> MGVVEEAHNVKVIGSGEATIVLGHGFGTDQSVWKHLVPHLVDDYRVVLYDNMGAGTTNPDYFDFDRYSNLEGYSFDLIAILEDLKIESCIFVGHSVSAMIGVLASLNRPDLFSKIVMISASPRYVNDVDYQGGFEQEDLNQLFEAIRSNYKAWCLGFAPLAVGGDMDSIAVQEFSRTLFNMRPDIALSVGQTIFQSDMRQILPFVTVPCHILQSVKDLVVPVVVSEYLHANLGCESVVEVIPSDGHLPQLSSPDSVIPVILRHIRNDIAM

A few components involved in KAR-signaling have been identified in Arabidopsis thaliana, including an α/β hydrolase fold protein, KARRIKIN INSENSITIVE2/HYPOSENSITIVE TO LIGHT (hereafter referred to as KAI2), an F-box protein, MORE AXILLARY GROWTH2 (MAX2, also referred to as ORESARA9/PLEIOTROPIC PHOTO SIGNALING/KARRIKIN INSENSITIVE1), and SUPPRESSOR OF MAX2 1 (SMAX1)/SMAX1-LIKE2 (SMXL2). Crystallographic studies and biochemical analyses have demonstrated the role of KAI2 as a KAR receptor. The structure of KAI2 displayed a canonical compact α/β-hydrolase domain that contained an α/β ‘core’ domain and a ‘lid’ domain. A smoke-derived compound, karrikin (KAR), and an endogenous but as yet unidentified KARRIKIN INSENSITIVE2 (KAI2) ligand (KL) have been identified as chemical cues in higher plants that impact on multiple aspects of growth and development.

Identification of the molecular lesion of the ply2 mutation revealed that it is a missense allele of KAI2 that causes an amino acid substitution, Ala219Val. Comparison of KAI2 and KAI2ply2 showed that there was little structural difference (r.m.s.d., 0.2 Å) in overall structure. However, in detail, we found that the residue A219 of KAI2 was bound to aromatic residues as Y124 and F134 of the lid domain by hydrophobic interactions, while the residue V219 of KAI2ply2 was bound to extended aromatic residues as Y124, F134, F157, F194, and H246 of the lid domain. Thus, the mutation Ala219Val caused stronger hydrophobic interactions with more residues. The entrance of KAI2 presents an opened pocket and hydrophobic charge for the ligand, whereas the entrance of KAI2ply2 forms a closed pocket due to C-gamma 1 and C-gamma 2 of V219, which is a bulkier residue than alanine. Thus, the narrowed entrance gate might contribute to the reduced ligand-binding ability of KAI2ply2. Furthermore, when we performed superimposition with the KAR1-bound KAI2 model previously reported by Guo et al. (2013), the V219 was predicted to cause a steric clash with the bound KAR. The results showed that the amino acid residues of KAI2 ranging from 125–150 exhibited a higher B-factor than those of KAI2ply2, implying that this region, corresponding to the helical ‘lid’ domain, might be more rigid with lower motional amplitude in the KAI2ply2 protein. The results suggested that KAI2ply2 was more thermally stable than the wild-type KAI2 protein, presumably due to increased hydrophobic interactions and reduced flexibility. Taken together, these results suggested that the Ala219Val substitution mutation of KAI2 not only impaired ligand-binding but also reduced the conformational flexibility of the lid domain, both of which would be critical for ligand perception and downstream signaling.>MSPILAKNIVYVAQIKGQITSYTYDQFDRYITIAEQDNAEAIIIELDTPGGRADAMMNIVQRIQQSKIPVIIYVYPPGASAAAAGTYIALGSHLIAMAPGTSIGACRPILGYSQNGSIIEAPPKITNYFIAYIKSLAQESGRNATIAEEFITKDLSLTPEEALKYG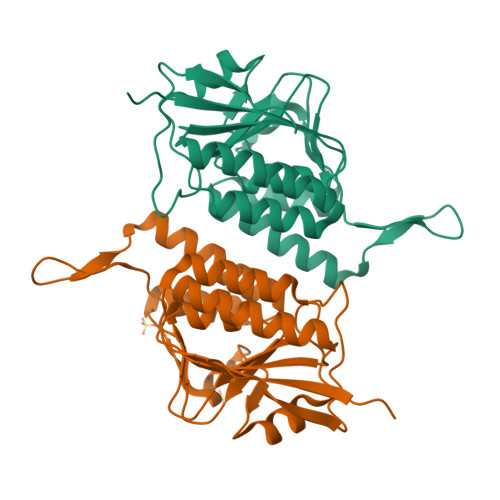VIEVVARDINELLKKSNGMKTKIPVNGRYVTLNFTNVEVRYLAPSFKDKLISYITDLEHHHHHH[2x]Here we describe an O-methyltransferase-like protein, AlpH, which is responsible for the hydrazine incorporation in kinamycin biosynthesis. AlpH catalyses a unique SAM-independent coupling of l-glutamylhydrazine and polyketide intermediate via a rare Mannich reaction in polyketide biosynthesis. Particularly, the O-methyltransferase (OMT)-like enzyme, AlpH, from the kinamycin BGC is determined to mediate the C-N bond formation through loading gluN2H3 to the polyketide scaffold. Biochemical assays and mutagenesis experiments demonstrated that AlpH catalyzes a SAM-independent Mannich reaction including hydrazine-carbonyl condensation and the following ring closure.

We determined the crystal structure of apo-AlpH to 1.87 Å resolution using the molecular replacement method, which exhibits a symmetric dimer conformation. Each AlpH monomer possesses 16 α-helixes (α1-α16) and 9 β-strands (β1−β9), forming two distinct sub-domains: an N-terminal dimerization domain and a C-terminal canonic α/β Rossmann fold catalytic domain. The swapped dimer conformation is mediated by the N-terminal dimerization domain of each AlpH monomer, which interlocks with each other and forms an extensive dimer interface, covering a total surface area of 3947 Å2. Structural comparison analyses of AlpH with LaPhzM and MmcR revealed an extra protruding N-terminal α−helix in AlpH that can further stabilize the interlocked dimer structure. However, PdxI possesses one more N-terminal α−helix comparing to AlpH for the formation of the swapped dimer. Notably, although the overall structure of the catalytic domain of AlpH shows high similarity to the SAM-dependent OMT LaPhzM and MmcR, there is no incorporation of SAM in the determined AlpH structure, in agreement with the previous finding that purified AlpH is free of SAM or SAH. Further structural comparison identified a unique solvent-exposed and negative charge enriched pocket between the dimerization domain and the catalytic domain in AlpH, which corresponds to the SAM/SAH binding pocket in MmcR28. Sequence alignment and structural comparison of the SAM/SAH binding pocket revealed that the critical glycine-rich GxGxG motif and F241 residue for SAH binding in MmcR/SAH complex are replaced by CxGxG and L252 residue in AlpH. Apparently, the bulky side chain of Cys introduces steric hindrance for SAM/SAH binding and the replacement of F241 by L252 also eliminates the putative π-π stacking interaction between SAM/SAH and the aromatic side chain of F241, leading to the reduced binding ability of AlpH for SAM/SAH. Given the uniqueness of the solvent-exposed pocket in AlpH, we propose that this pocket might be the substrate-binding pocket to generate 9. Intriguingly, the loss of SAM binding is critical for AlpH, providing an additional binding site for gluN2H3.

>[2x]MPELPPPHVVREAEKARADLQRQSRELAPPPFALLELIMGVMVTRAVHVAAELKVAEALAEGPLSADELAGRVGADADALGRVLRLLASNGVFATRPDGAFELTPMADALRADHPMSMRGIALLMGHPIHWEDWSGFPETVVTGEPALPKLRGMHAFEFLTKNAEYGQVFFQGMGSMSASETEPILAAYDFSQFGTVVDFCGGQGALLAGILGAAPGCEGVLFDPRVEENGAAEFLAAQGVADRTKRVAGDLFDVPPGGADAYVLKHIVHDWPEEQALRILRNVRAAIKPGGKLLIAEMVIPEQGDQPHSGKLVDLWLMLLVGGRERTPGQYADLLARAGFRLERVVETAAAISLVEAVPV>[2x]SSGNFILTHITSHNWSTIFSLLGPKKFLELLVNNKGFVSKVNGESVQIFGDVNSHRKAVVVSKYITKFNVLYNSYSRDFSRFEMIRPSIQTILQDILSFSGLNPGRSSKRYRGFKSLLSRIIANDKKCRYDILYAKFIGTSKCNFANVVSNKTEISQVIQFVLLVLGKLLPLDAWGGVSNKKIIKDRVVDFLLLGANEKIHMDDLFRGIRLKDFKWLGRAHQISSKQDFELRTAFLKGYLWWLFEHLLKNILRSFWYITETSSIVSLELNYFPQYLWKELYESWVSKYAKNNLVKMPSKIQREQLPCGKIKLIPKRSSFRVICVPIKRSLKLLNKKLELDTLEKEKREFERYRKEVLSPVGQILRLKLSKLRDTYESYRASVHSSSDVAEKISDYRDSLLTRFGEIPKLFILKFDMKECYDRLSQPVLMKKLEELFENQDNKTSYYVRYYAQLDASHKLKKVKTTIDTQYHNLNILSSSRHLSNCKSLVDKTKTI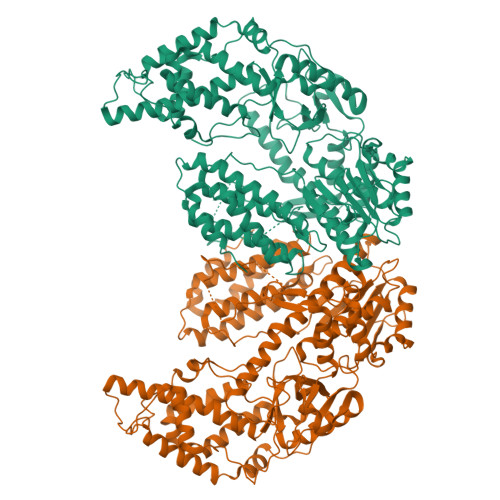ALQKGNILEVCRSQIYDVVGSVKDARGNLHLYKRKRGVFQGFSLSSIFCDILYSAMVHDCFQFLWKSKQDFLFVRLVDDFLLVTPDSNIYDQVHNILSGKILESYGAFVNKDKTVVVNQTTTKPSIDFVGLEVNTTDLSIKRNSGSISLVTTNFRTFKTLVKYLKTFYQLNLEGFLLDCSFGVLENVLENMGSLLRLVLREFKTKFTSIVKYDTFHCYKFIKFLYDISNYTIVKYVETNSDWDGAPELLNCIKQIIVKEFSSFESYSEIVEWVQTLNI>MESPEEPGASMDENYFVNYTFKDRSHSGRVAQGIMKLCLEEELFADVTISVEGREFQLHRLVLSAQSCFFRSMFTSNLKEAHNRVIVLQDVSESVFQLLVDYIYHGTVKLRAEELQEIYEVSDMYQLTSLFEECSRFLARTVQVGNCLQVMWLADRHSDPELYTAAKHCAKTHLAQLQNTEEFLHLPHRLLTDIISDGVPCSQNPTEAIEAWINFNKEEREAFAESLRTSLKEIGENVHIYLIGKESSRTHSLAVSLHCAEDDSISVSGQNSLCHQITAACKHGGDLYVVGGSIPRRMWKCNNATVDWEWCAPLPRDRLQHTLVSVPGKDAIYSLGGKTLQDTLSNAVIYYRVGDNVWTETTQLEVAVSGAAGANLNGIIYLLGGEENDLDFFTKPSRLIQCFDTETDKCHVKPYVLPFAGRMHAAVHKDLVFIVAEGDSLVCYNPLLDSFTRLCLPEAWSSAPSLWKIASCNGSIYVFRDRYKKGDANTYKLDPATSAVTVTRGIKVLLTNLQFVLA[2x];> MAYSQGGGKKKVCYYYDGDIGNYYYGQGHPMKPHRIRMTHNLLLNYGLYRKMEIYRPHKATAEEMTKYHSDEYIKFLRSIRPDNMSEYSKQMQRFNVGEDCPVFDGLFEFCQLSTGGSVAGAVKLNRQQTDMAVNWAGGLHHAKKSEASGFCYVNDIVLAILELLKYHQRVLYIDIDIHHGDGVEEAFYTTDRVMTVSFHKYGEYFPGTGDLRDIGAGKGKYYAVNFPMRDGIDDESYGQIFKPIISKVMEMYQPSAVVLQCGADSLSGDRLGCFNLTVKGHAKCVEVVKTFNLPLLMLGGGGYTIRNVARCWTYETAVALDCEIPNELPYNDYFEYFGPDFKLHISPSNMTNQNTPEYMEKIKQRLFENLRMLPHAPGVQMQAIPEDAVHEDSGDEDGEDPDKRISIRASDKRIACDEEFSDSEDEGEGGRRNVADHKKGAKKARIEEDKKETEDKKTDVKEEDKSKDNSGEKTDTKGTKSEQLSNP

Kelch repeat and BTB domain-containing protein 4 (KBTBD4) is the substrate receptor of a cullin3-dependent E3 ligase complex (CRL3KBTBD4). Recurrent indel mutations in the Kelch domain of the KBTBD4 E3 ligase rewire epigenetic programs for stemness in medulloblastoma by recruiting LSD1-CoREST-HDAC1/2 complexes as neo-substrates for ubiquitination and degradation. UM171, an investigational drug for haematopoietic stem cell transplantation, was found to degrade LSD1-CoREST-HDAC1/2 complexes in a wild-type KBTBD4-dependent manner, suggesting a potential common mode of action. The mutant and drug-induced complexes adopt similar structural assemblies requiring both Kelch domains in the KBTBD4 dimer for each HDAC2 interaction.

To determine the structure of the lower affinity KBTBD4WT complex mediated by UM171, we used the BS3 crosslinker to stabilise the binding of the CoREST1NT2-HDAC2 neo-substrate. This sample yielded 2:2 and 2:1 KBTBD4WT-UM171-HDAC2 complexes at 2.9 Å and 3.1 Å, respectively. The cryo-EM datasets for the KBTBD4WT-UM171-HDAC2 complexes yielded 2:1 and 2:2 models displaying an RSMD value of 1.55 Å across 1055 Cα positions. Superposition of the 2:1 and 2:2 states shows that the high structural conservation extends across the protein-compound and protein-protein interaction sites, indicating that the neo-substrate recruitment mechanism in these complexes is conserved regardless of the stoichiometry. The asymmetric 2:1 and 2:1:1 models allowed comparison of the equivalent KBTBD4WT site 1 in both the bound and unbound states. Interestingly, UM171 was only observed in the HDAC2-bound site 1 and not in the second Kelch domain, suggesting that UM171 binding requires both proteins to be present. Notably, UM171 binding exhibited an induced-fit mechanism requiring the opening of a cleft between Kelch domain blades II and III to accommodate the benzyl group of UM171. In the UM171-bound KBTBD4WT protomer, L356 (BC III loop) is shifted a further 3.4 Å away from P311 (BC II loop) and 4.1 Å from L335 (DA III loop) relative to the unbound site 1 in the other KBTBD4WT protomer. Similar to site 1, site 2 in the 2:1 model shows subtle conformational changes between the HDAC2-bound and unbound states. In particular, KBTBD4WT L406 in the BC IV loop shows a shift of 6.9 Å to pack together with KBTBD4WT F408 and F409 into a shallow hydrophobic pocket on the HDAC2 surface.>ETQELASKRVDIQNKRFYLDVKQNAK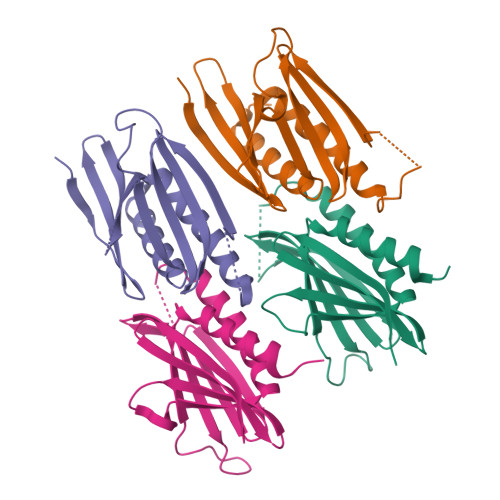GRFLKIAEVGAGGNKSRLTLSMSVAVEFRDYLGDFIEHYAQLGPSQPPDLAQAQDEPPRALKSEFLVRENRKYYMDLKENQRGRFLRIRQTVNRGPGLGSTQGQTIALPAQGLIEFRDALAKLIDDYGVE[4x]> MSSQKVFGITGPVSTVGATAAENKLNDSLIQELKKEGSFETEQETANR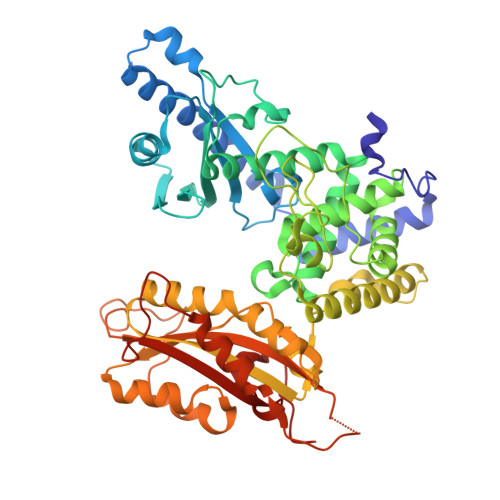VQVLKILQELAQRFVYEVSKKKNMSDGMARDAGGKIFTYGSYRLGVHGPGSDIDTLVVVPKHVTREDFFTVFDSLLRERKELDEIAPVPDAFVPIIKIKFSGISIDLICARLDQPQVPLSLTLSDKNLLRNLDEKDLRALNGTRVTDEILELVPKPNVFRIALRAIKLWAQRRAVYANIFGFPGGVAWAMLVARICQLYPNACSAVILNRFFIILSEWNWPQPVILKPIEDGPLQVRVWNPKIYAQDRSHRMPVITPAYPSMCATHNITESTKKVILQEFVRGVQITNDIFSNKKSWANLFEKNDFFFRYKFYLEITAYTRGSDEQHLKWSGLVESKVRLLVMKLEVLAGIKIAHPFTKPFESSYCCPTEDDYEMIQDKYGSHKTETALNALKLVTDENKEEESIKDAPKAYLSTMYIGLDFNIENKKEKVDIHIPCTEFVNLCRSFNEDYGDHKVFNLALRFVKGYDLPDEVFDENEKRPSKKSKRKN> EREKLLRLEEELHKRVVGQDEAIRAVADAIRRARAGLKDPNRPIGSFLFLGPTGVGKTELAKTLAATLFDTEEAMIRIDMTEYMEKHAVSRLIGAPPGYVGYEE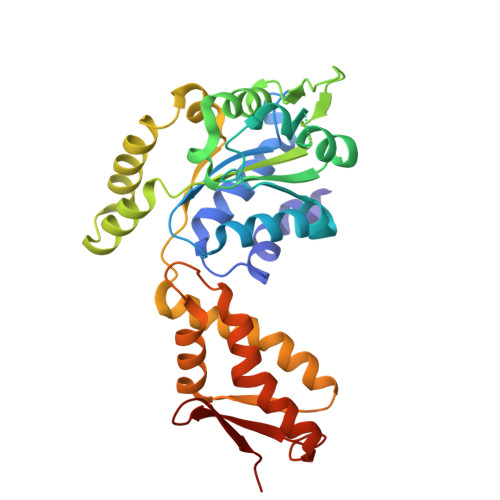GGQLTEAVRRRPYSVILFDAIEKAHPDVFNILLQILDDGRLTDSHGRTVDFRNTVIILTSNLGSPLILEGLQKGWPYERIRDEVFKVLQQHFRPEFLNRLDEIVVFRPLTKEQIRQIVEIQLSYLRARLAEKRISLELTEAAKDFLAERGYDPVFGARPLRRVIQRELETPLAQKILAGEVKEGDRVQVDVGPAGLVFAVPARV> GKENEENIQCGENFMDIECFMVLNPSQQLAIAVLSLTLGTFTVLENLLVLCVILHSRSLRCRPSYHFIGSLAVADLLGSVIFVYSFIDFHVFHRKDSRNVFLFKLGGVTASFTASVGSLFLAAIDRYISIHRPLAYKRIVTRPKAVVAFCLMWTIAIVIAVLPLLGWNCEKLQSVCSDIFPHIDETYLMFWIGVTSVLLLFIVYAYMYILWKAGIDCSFWNESYLTGSRDERKKSLLSKFGMDEGVTFMFIGRFDRGQKGVDVLLKAIEILSSKKEFQEMRFIIIGKGDPELEGWARSLEEKHGNVKVITEMLSREFVRELYGSVDFVIIPSYFEPFGLVALEAMCLGAIPIASAVGGLRDIITNETGILVKAGDPGELANAILKALELSRSDLSKFRENCKKRAMSFSDQARMDIRLAKTLVLILVVLIICWGPLLAIMVYDVFGKMNKLIK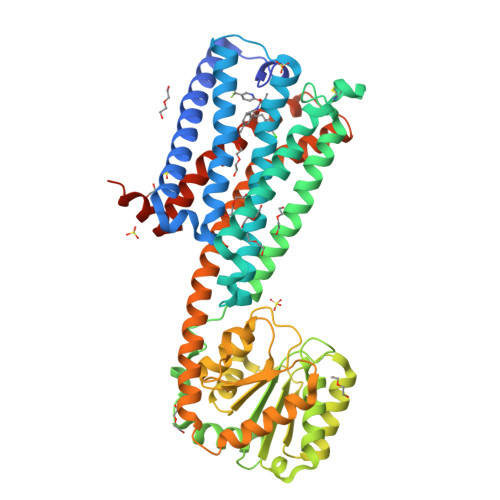TVFAFCSMLCLLNSTVNPIIYALRSKDLRHAFRSMFPSCEGTAQPHHHHHHHHHH>[8x]GGGRSPSLPTQTCGPWEMKERLGTGGFGYVLRWIHQDTGEQVAIKQCRQELSPKNRERWCLEIQIMKKLNHPNVVSAREVPDGLQKLAPNDLPLLAMEYCEGGDLRKYLNQFENCCGLKEGPIRTLLSDISSALRYLHENRIIHRDLKPENIVLQPGPQRLIHKIIDLGYAKELDQGELCTEFVGTLQYLAPELLEQKKYTVTVDYWSFGTLAFECITGFRPFLPNWQPVQWHGKVREKSNEHIVVYDDLTGAVKFSSVLPTPNHLSGILAGKLERWLQCMLMWHQRQRGTDPQNPNVGCFQALDSILSLKLLSVMNMVSGRVHTYPVTENENLQNLKSWLQQDTGIPEEEQELLQASGLALNSAQPLTQYVIDCTVIDGRQGEGDLIFLFDNRKTVYEPQISLPAHPESVSIVLQDPKRPLTYTHLRRVWGQIWQTIRALK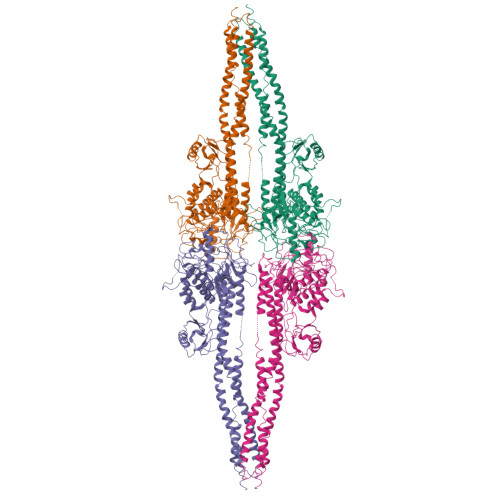EDCARLLQGQRTSMVNLLRYNTELSKKKNSMTSECEQLKAKLDFFRSSIQIDLEKYSEQMEFGITSEKLLSAWREMEQAVELCGREREVQALVDKMMALQTDSVDLQRNPLGRKHRGTLDDLEEQARDLYRRLRERPRDQRTPGDSNDMVRLLILAIQSFEKRVILIYDQLSKTVVCKRKALELSPKVKEVMNLMREDEKIVVRRQEKRQQELWNLLKIACSKVRGPVSGSPDS>MRLSELKTGEKGVIVKVLGHGGFRKRIVEMGFIKGKTVEVLLNAPLKDPIKYKIMGYEISLRRQEADMIEIISEQE[2x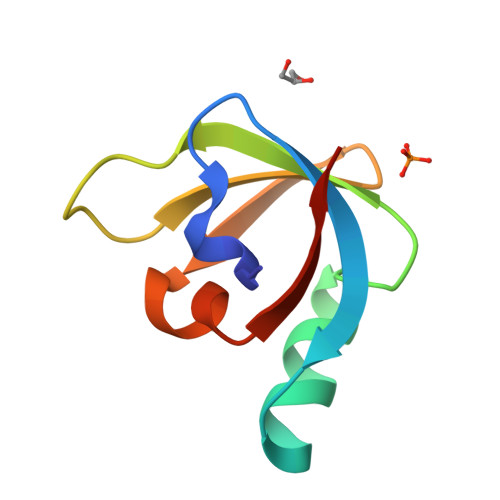]>[6x]SPNIKIFSGSSHQDLSQKIADRLGLELGKVVTKKFSNQETCVEIGESVRGEDVYIVQSGCGEINDNLMELLIMINACKIASASRVTAVIPCFPYARQDKKDKSRAPISAKLVANMLSVAGADHIITMDLHASQIQGFFDIPVDNLYAEPAVLKWIRENISEWRNCTIVSPDAGGAKRVTSIADRLNVDFALIHKERKKANEVDR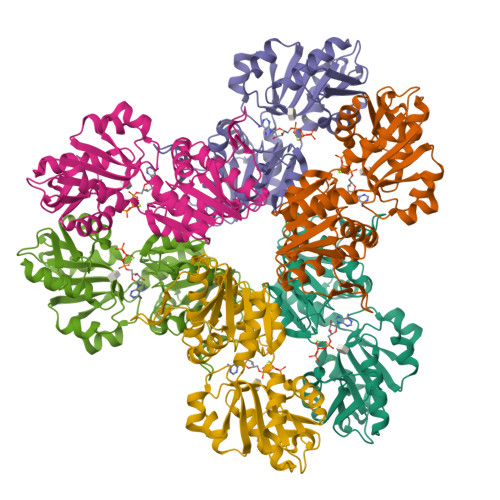MVLVGDVKDRVAILVDDMADTCGTICHAADKLLSAGATRVYAILTHGIFSGPAISRINNACFEAVVVTNTIPQEDKMKHCSKIQVIDISMILAEAIRRTHNGASVSYLFSHVPL> NRIITEYILIDANNYHFKSWIECFPDCKVNLKLLLFRPEWFDF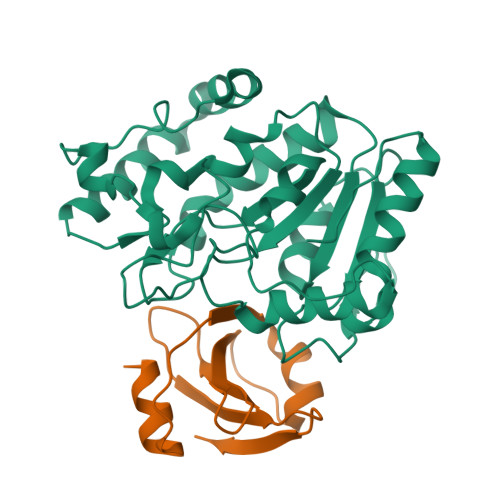FKYVESKTYFPQLESKLSSYLEKRQRIVPYPELLFNTMNVLPPGKIKVVILGQDPYPGSCISGVPYAMGCSFSVPLNCPVPKSLANIYTNLIKFNHMRKAPKHGCLASWILQGTFMINSAFTTVLNESGVHARTWESFTADLIDYLTDNYDDLIFVAWGAHAHKLCQRVDPKKHYIITSSHPSPFSVSNTMTSMSYGPNPKKVTYPSFNSVDHFGKINEHLKSRNKKPIFWDL;> TNLSDIIEKETGKQLVIQESILMLPEEVEEVIGNKPESDILVHTAYDESTDENVMLLTSDAPEYKPWALVIQDSNGENKIKML>MSAASWSHPQFEKMSRDEVESLIQEVLEVYPEKAKKNREKHLSPNDPELEQSKKCITSNKKSLPGVMTIRGCAYAGSKGVVWGPIKDMIHISHGPVGCGQYSRAGRRNYYIGTTGVNAFVTMNFTSDFQEKDIVFGGDKKLAKLIDEIETLFPLNKGISVQSECPIGLIGDDIEAVSKQKGKEHGKTIVPVRCEGFRGVSQSLGHHIANDAVRDWVLSARDDDDSFETTDYDVAIIGDYNIGGDAWSSRILLEEMGLRVVAQWSGDGTISEMELTPKVKLNLVHCYRSMNYISRHMEEKYGIPWMEYNFFGPTKTIESLRKIAAQFDESIQKKCEEVIAKYQPEWEAVVAKYRPRLEGKRVMLYVGGLRPRHVIGAYEDLGMEVVGTGYEFGHNDDYDRTLKEMGDSTLLYDDVTGYEFEEFVKKVKPDLIGSGIKEKYIFQKMGIPFRQMHSWDYSGPYHGFDGFAIFARDMDMTLNNPCWKKLQAPWKKSEQADEAVAASA[2x];>[2x]MSQQVDKIKASYPLFLDQDYKDMLAKKRDGFEEKYPQDKIDEVFQWTTTKEYQELNFQREALTVNPAKACQPLGAVLCALGFEKTMPYVHGSQGCVAYFRSYFNRHFREPVSCVSDSMTEDAAVFGGQQNMKDGLQNCKATYKPDMIAVSTTCMAEVIGDDLNAFINNSKKEGFIPDEFPVPFAHTPSFVGSHVTGWDNMFEGIARYFTLKSMDDKVVGSNKKINIVPGFETYLGNFRVIKRMLSEMGVGYSLLSDPEEVLDTPADGQFRMYAGGTTQEEMKDAPNALNTVLLQPWHLEKTKKFVEGTWKHEVPKLNIPMGLDWTDEFLMKVSEISGQPIPASLTKERGRLVDMMTDSHTWLHGKRFALWGDPDFVMGLVKFLLELGCEPVHILCHNGNKRWKKAVDAILAASPYGKNATVYIGKDLWHLRSLVFTDKPDFMIGNSYGKFIQRDTLHKGKEFEVPLIRIGFPIFDRHHLHRSTTLGYEGAMQILTTLVNSILERLDEETRGMQATDYNHDLVR

Nitrogenase provides access to bioessential nitrogen via the reduction of highly inert atmospheric dinitrogen (N2) to ammonia (NH3). In all nitrogenase isozymes, H-subunits form a homodimeric reductase component (‘HH’) that transiently associates with and transfers electrons to a catalytic core. This catalytic component is a heterotetramer composed of two D- and two K-subunits (‘DDKK’ or α2β2) and contains the active site metallocluster where N2 is bound and reduced to NH3. Three previously characterized ancestral variants were targeted from phylogenetic nodes within the evolutionary lineage of Azotobacter vinelandii Nif (wild-type, ‘WT’) (Garcia et al., 2023): Anc1A, Anc1B, and Anc2.

Anc1A and Anc1B are the same age, whereas Anc2 is reconstructed from an older phylogenetic node. As an additional distinction, Anc1A and Anc2 contain an ancestral D-subunit protein complexed with WT H- and K-subunit proteins. Specifically, all ancestors crystallized at pH 6.5, which is unusually acidic for nitrogenase. In addition, all ancestral proteins crystallized in space group P 212121, which differs from the space groups for the same proteins in A. vinelandii NifDK (i.e., WT; space group P 21), Clostridium pasteurianum Nif (space group P 21), and Klebsiella pneumoniae NifDK (space group C 2). All three ancestors showed anisotropic diffraction: 2.65–2.93 Å for Anc1A, 1.82–2.8 Å for Anc1B, and 1.82–2.42 Å for Anc2. Global structural differences between the ancestors and WT A. vinelandii DDKK are relatively minor and within the range of variation for available extant structures. Among the two hybrid ancestors, the RMSD between Anc2 and WT (0.24 Å) is smaller than that between Anc1A and WT (0.31 Å). Notably, a non-conserved Nif-D α-helix (positions 165–174 in Anc1B) lies within interacting distance of HH. This helix contains several substitutions across all ancestors, albeit the positioning of polar amino acids differs among Anc1A, Anc1B, and Anc2. Herein, the D-subunit S165A substitution is consistently present across all ancestors and may influence interactions with HH S175 in the ATP-bound complex, potentially reducing stability.> XPPGPPGPPGPRGLPGPPGPP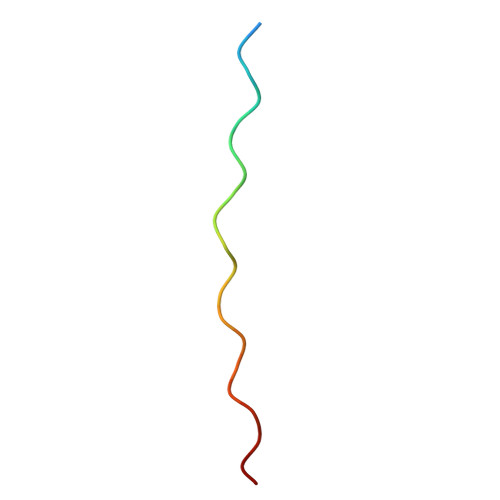G>MAHHHHHHMFDVVISDIEAREILDSRGYPTLCVKVITNTGTFGEACVPSGASTGIKEALELRDKDPKRYQGKGVLQAISNVEKVLVPALQGFSVFDQITADAIMIDADGTPNKEKLGANAILGVSLALAKAAANTLQRPLYRYLGGSFSHVLPCPMMNLINGGMHATNGLQFQEFMIRPISAPSLKEAVRMGAEVFNALKKILQNRQLATGVGDEGGFAPNLASNAEALDLLLTAIETAGFTPREDISLALDCAASSFYNTQDKTYDGKSYADQVGILAELCEHYPIDSIEDGLAEEDFEGWKLLSETLGDRVQLVGDDLFVTNSALIAEGIAQGLANAVLIKPNQIGTLTETAEAIRLATIQ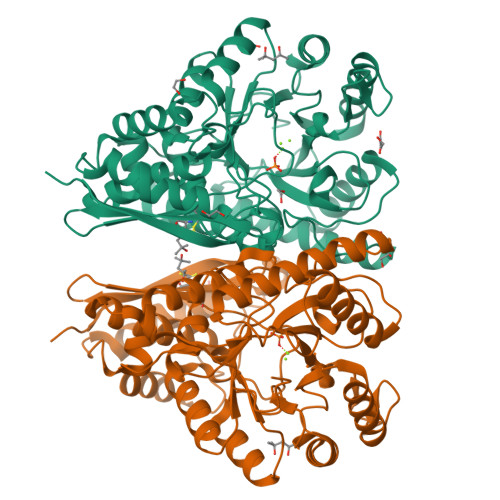GYATILSHRSGETEDTTIADLAVAFNTGQIKTGSLSRSERIAKYNRLMAIEEEMGPEALFQDSNPFSKA[2x]> DEPK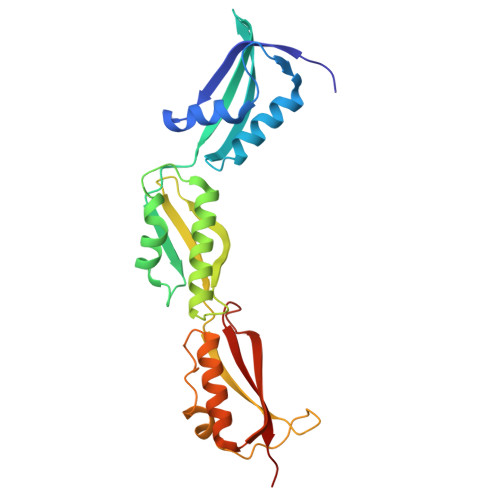VLIAEVVVEGATPELEQLVYQVISTRPGSTTTRTQLQQDTNAIFATGFFADVNAVPRDTPLGVRITFVVRPYPVLRAVQVAGNQVLTQEKVNEIFAPQIGRTLNLRELQAGIEKINTFYRDNGYILGQVVGTPQVDPDGVVTLQVAEGVVEQVTYRFLNKEGEPTKQRTRDFVISREMDTQPGVVLNQKTVQADLRRLFELGLFEDVQVALEPGQNPRRVNLILNIKERNT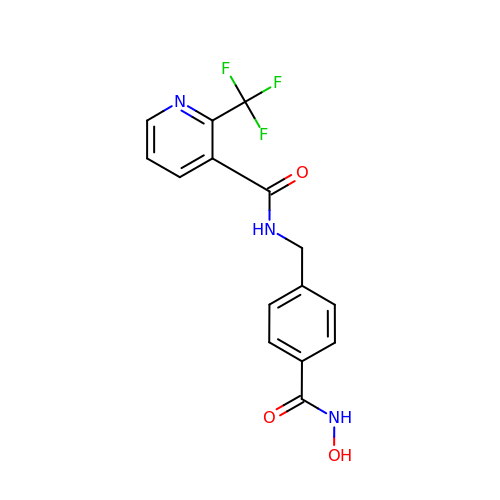N-{[4-(hydroxycarbamoyl)phenyl]methyl}-2-(trifluoromethyl)pyridine-3-carboxamide | C15 H12 F3 N3 O3 | SQBRKYYJEYSFMY-UHFFFAOYSA-N The OXA-48 carbapenemase is widely disseminated in Enterobacterales, necessitating new treatments for producer strains. OXA-48 is a class D SBL that uses a nucleophilic serine (Ser70) to hydrolyse β-lactams, with a proximal post-translationally carbamylated lysine (Lys73) proposed to act as the general base for both the acylation and deacylation steps of the reaction. Diazabicyclooctane (DBO) inhibitors, including avibactam and nacubactam, act on a wide range of enzymes to overcome β-lactamase-mediated resistance. Here we describe investigations on how avibactam and nacubactam inhibit OXA-48 and two variants, OXA-163 and OXA-405, with deletions in the β5–β6 loop neighbouring the active site that modify activity towards different β-lactam classes.

We determined high-resolution crystal structures of uncomplexed, avibactam- and nacubactam-bound OXA-48, OXA-163 and OXA-405 to investigate how differences in the β5–β6 loop composition relate to DBO potency. To investigate the possibility that the differences between avibactam and nacubactam binding affect the dynamic behaviour of OXA-48, molecular mechanics molecular dynamics (MM MD) was used to simulate uncomplexed, avibactam- and nacubactam-bound OXA-48. In contrast, such differences are less prominent when the avibactam-bound structure is compared with that of uncomplexed OXA-48, although the Arg214 RMSF increases slightly in the former. In contrast, in the avibactam-bound or uncomplexed structures the t-rotamer is preferred. Val120, the other residue contributing to the OXA-48 deacylating water channel, consistently adopts the t-rotamer, as observed in the crystal structures, in all simulations of the uncomplexed and DBO-bound enzyme. Arg214 is considered to contribute to the carbapenemase activity of OXA-48, possibly through its stabilisation of the Ω-loop, modifications to the active site electric field and/or hydration.

>[2x]GPKEWQENKSWNAHFTEHKSQGVVVLWNENKQQGFTNNLKRANQAFLPASTFKIPNSLIALDLGVVKDEHQVFKWDGQTRDIATWNRDHNLITAMKYSVVPVYQEFARQIGEARMSKMLHAFDYGNEDISGNVDSFWLDGGIRISATEQISFLRKLYHNKLHVSERSQRIVKQAMLTEANGDYIIRAKTGYSTRIEPKIGWWVGWVELDDNVWFFAMNMDMPTSDGLGLRQAITKEVLKQEKIIP> AVKYYTLEEIQKHNNSKSTWLILHYKVYDLTKFLEEHPGGEAVLREQAGGDATANFEDVGHSTDARELSKTFIIGELHPD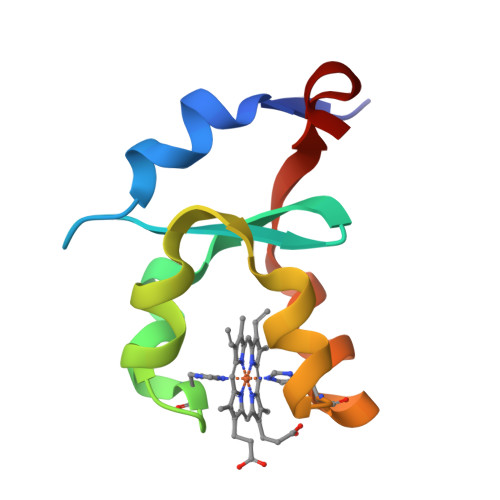DR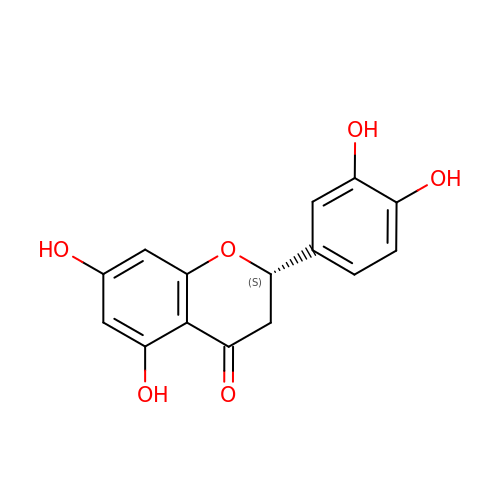(2S)-2-(3,4-DIHYDROXYPHENYL)-5,7-DIHYDROXY-2,3-DIHYDRO-4H-CHROMEN-4-ONE | C15 H12 O6 | SBHXYTNGIZCORC-ZDUSSCGKSA-N> ASMTGGQQMGRDEAGITGTWYNQLGSTFIVTAGADGALTGTYESAVGNAESRYVLTGRYDSAPATDGSGTALGWTVAWKNNYRNAHSATTWSGQYVGGAEARINTQWLLTIGTTEANAWRSTLVGHDTFTKVKP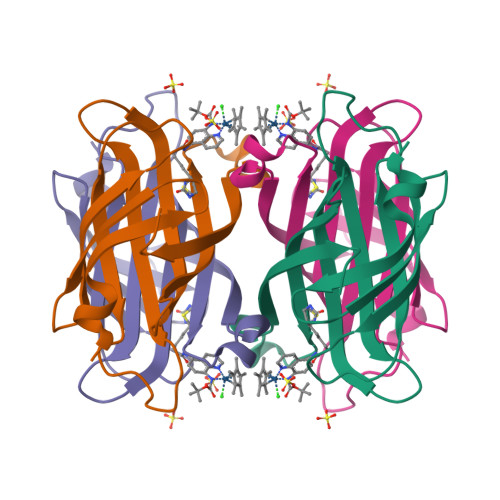SAASIDAAKKAGVNNGNPLDAVQQ>MNDQPFAWQVASLSERYQEQFDIGAAVEPYQLEGRQAQILKHHYNSLVAENAMKPESLQPREGEWNWEGADKIVEFARKHNMELRFHTLVWHSQVPEWFFIDEDGNRMVDETDPDKREANKQLLLERMENHIKTVVERYKDDVTSWDVVNEVIDDGGGLRESEWYQITGTDYIKVAFETARKYGGEEAKLYINDYNTEVPSKRDDLYNLVKDLLEQGVPIDGVGHQSHIQIGWPSIEDTRASFEKFTSLGLDNQVTELDMSLYGWPPTGAYTSYDDIPAELLQAQADRYDQLFELYEELAADISSVTFWGIADNHTWLDGRAREYNNGVGIDAPFVFDHNYRVKPAYWRIIDLEHHHHHH[2x]

Xylanase [EC 3.2.1.8] hydrolyzes the internal β-1,4-linkage of xylan. A GH10 xylanase XynR was identified in the culture broth of TAR-110. GH10 xylanases have a (β/α)8 triose-phosphate isomerase (TIM) barrel fold while GH11 xylanases have a β-jellyroll fold composed of eight β strands. GH10 and GH11 xylanases have two conserved catalytically important E residues in the active site.

To explore the role of this extended loop on the substrate binding and catalytic activity, we made crystallographic analysis of WT complexed with xylobiose. The space group of the crystal was P21, and the structure was refined at 1.80 Å resolution. The whole structure of WT complexed with xylobiose exhibited no difference compared to ligand-free WT13 with rmsd of 0.21 Å for 353 Cα atoms in chain A. Figure 7A shows the active-site structure of WT complexed with xylobiose, and Fig. 7B shows the comparison of WT and T315Q. In the region (residue 311–331) with the largest deviation between T315Q and WT, three residues (D312, D318, and D331) are involved in the Ca2+ binding, and two residues are involved in the binding to xylobiose. R320 interacts with O5 of subsite + 1 xylose and O3 of subsite + 217, and is located near the acidic and basic catalytic residues (E150 and E256, respectively) with 8.0 and 8.8 Å, respectively. These evidences suggest that the mutation of T315 to Q deviates the position of R320, affecting the dissociation of E150, leading to increase in alkaliphily of T315Q.>MHHHHHHGSDDDDKRPEAKSAQPADGWKGERPRSEEDNELNLPNLAAAYSSILSSLGENPQRQGLLKTPWRAASAMQFFTKGYQETISDVLNDAIFDEDHDEMVIVKDIDMFSMCEHHLVPFVGKVHIGYLPNKQVLGLSKLARIVEIYSRRLQVQERLTKQIAVAITEALRPAGVGVVVEATHMCMVMRGVQKMNSKTVTSTMLGVFREDPKTREEFLTLIRS[5x]

Guanosine triphosphate (GTP) cyclohydrolase I (GCH1) (EC:3.5.4.16) catalyzes the conversion of GTP to dihydroneopterin triphosphate (H2NTP). This reaction is the first and rate-limiting step involved in the de novo synthesis of tetrahydrobiopterin (BH4). The effects of GFRP on GCH1 occur via formation of heteromeric protein complexes between GCH1 and GFRP, which are dependent on the intracellular concentrations of the effector molecules phenylalanine or BH4. GCH1−GFRP complexes consist of one GCH1 decamer flanked by two pentameric GFRP complexes.

We determined structures of the human GCH1 in the absence (xtal_GCH1) and presence (xtal_GCH1+active) of the substrate analog 7-deaza-GTP and in the presence of the allosteric inhibitor cpd-1 (xtal_GCH1+allosteric and xtal_GCH1+allosteric). Xtal_GCH1 is a redetermination of the previously determined apo-hGCH1 structure. For the unliganded form xtal_GCH1, weak electron density is visible for region A that allows for tracing the main chain, suggesting that a partially flexible region A is a signature of the basally active state of GCH1. This degree of flexibility in region A, which could possibly serve as a lid for the active site, could be essential to allow substrate association. Region B consisting of residues 213 to 222 is only weakly defined in the electron densities in all structures without an active site ligand bound (xtal_GCH1, EM_GCH1+hGFRP+allosteric, and xtal_GCH1+allosteric).(3S,6S)-3,6-bis(2-methylpropyl)piperazine-2,5-dione | C12 H22 N2 O2 | 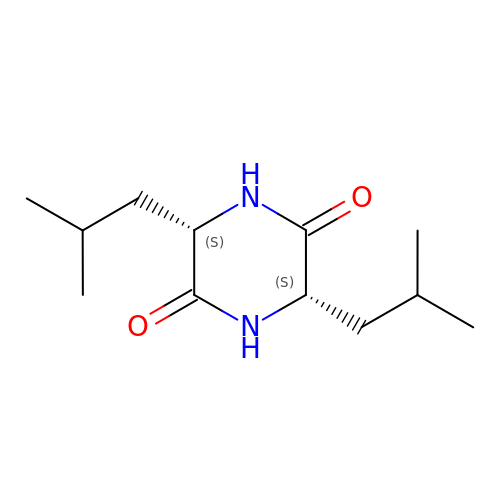XWYXUMDVQIOAPR-UWVGGRQHSA-N>[4x]MHHHHHHSSGRENLYFQGEVDMHPPLPQPVHPDVTMKPLPFYEVYGELIRPTTLASTSSQR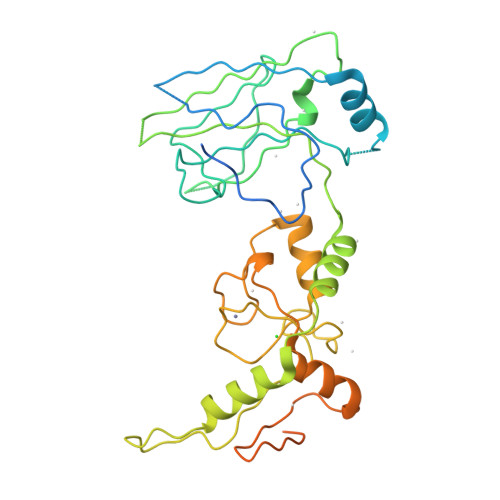FEEAHFTFALTPQQVQQILTSREVLPGAKCDYTIQVQLRFCLCETSCPQEDYFPPNLFVKVNGKLCPLPGYLPPTKNGAEPKRPSRPINITPLARLSATVPNTIVVNWSSEFGRNYSLSVYLVRQLTAGTLLQKLRAKGIRNPDHSRALIKEKLTADPDSEVATTSLRVSLMCPLGKMRLTVPCRALTCAHLQSFDAALYLQMNEKKPTWTCPVCDKKAPYESLIIDGLFMEILSSCSDCDEIQFMEDGSWCPMKPKKEASEVCPPPGYGLDGLQYSPVQGGDPSENKKKVEVIDLTIESSSDEEDLPPTKKH> APAVADKADNAFMMICTALVLFMTIPGIALFYGGLIRGKNVLSMLTQVTVTFALVCILWVVYGYSLAFGEGNNFFGNINWLMLKNIELTAVMGSIYQYIHVAFQGSFACITVGLIVGALAERIRFSAVLIFVVVWLTLSYIPIAHMVWGGGLLASHGALDFAGGTVVH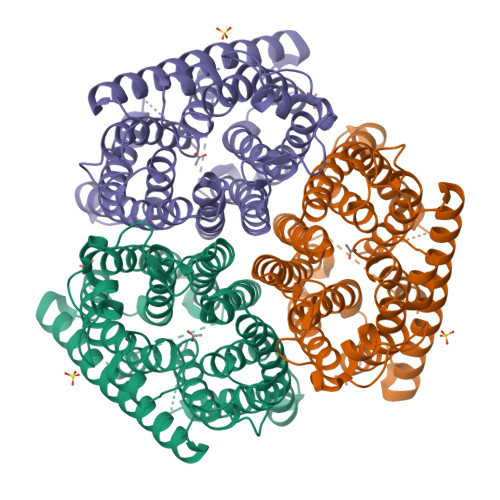INAAIAGLVGAYLIGKRVGFGKEAFKPHNLPMVFTGTAILYIGWFGFNAGSAGTANEIAALAFVNTVVATAAAILGWIFGEWALRGKPSLLGACSGAIAGLVGVTPACGYIGVGGALIIGVVAGLAGLWGVTMLKRLLRVDDPCDVFGVAGVCGIVGCIMTGIFAASSLGGVGFAEGVTMGHQLLVQLESIAITIVWSGVVAFIGYKLADLTVGLRVPEEQEREGLDVNSHGENAYNADQAQQPAQADLEHHHHHH>MGSHHHHHHSSGENLYFQGHMVFGMLLLSRSDLEKLISMKEVIESVERAFLELYNGKAKVPLRTIIEV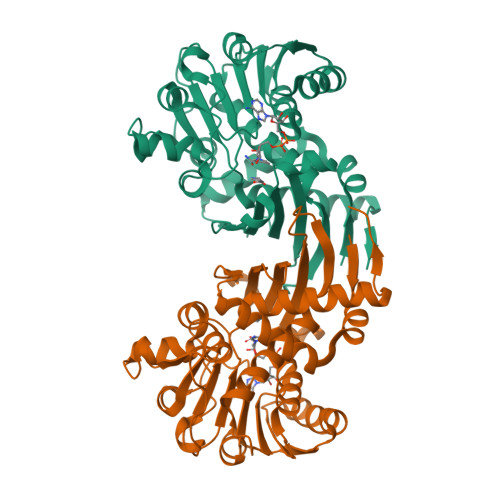EKHNGFILYMPSYLEDSEALAVKVVSLYPENTKKGLPSVLASILLNDPKTGAPLALMEGTFITAMRTGAASGVATKYLARKDSKIAGIIGAGVQARTQLWAVCEVRNIEKALVYDINPKNAKKFAEEMSKKLGIEIKTVESAREATEKSDILIVATTAREPVVKGGWIREGTHINSVGWVGRDARELDSETVRKSKLVVDSKEGVLNESGDIIIPMKEGVIDEGHIHAELAEIVAGVKKGRENNREITLFKSVGLAIEDAITAKLAYEKALEHGVGTNVEL[2x]>[2x]IPEYVDWRQKGAVTPVKNQGSCGSCWAFSAVVTIEGIIKIRTGNLNEYSEQELLDCDRRSYGCNGGYPWSALQLVAQYGIHYRNTYPYEGVQRYCRSREKGPYAAKTDGVRQVQPYNEGALLYSIANQPVSVVLEAAGKDFQL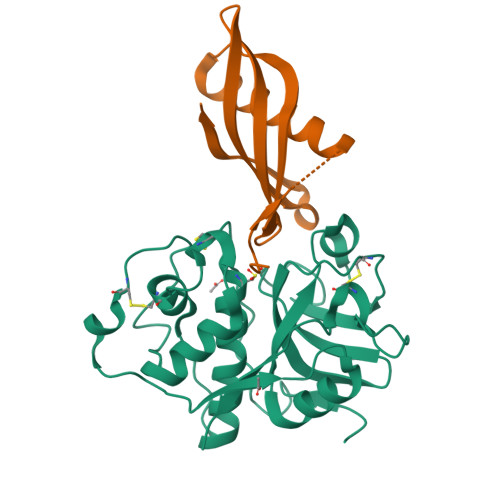YRGGIFVGPCGNKVDHAVAAVGYGPNYILIKNSWGTGWGENGYIRIKRGTGNSYGVCGLYTSSFYPVKN;>ALMGGIVDVEGAQNSAEVEELARFAVDEHNKKENALLQFSRLVKAKQQVVSGIMHHLTVEVIEGGKKKVYEAKVWVQAWLNSKKLHEFSPI[2x]~{N}-(3-methoxy-4-methyl-phenyl)-4-(4-methoxy-2-oxidanylidene-3~{H}-benzimidazol-1-yl)piperidine-1-carboxamide 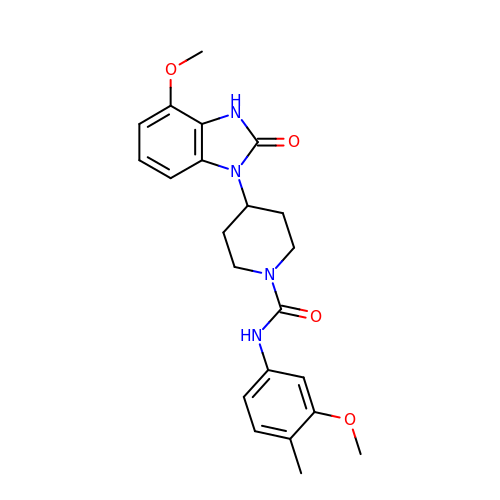| C22 H26 N4 O4 | CPZCKKAMAVISMR-UHFFFAOYSA-N>MHVRDTKLTVDDITGVVGIIPTPSIPTADQPGTAFSVDLDEAATLADAMVRGGVDVLMTTGTFGECASLTWDELQSFVATVVDAVAGRIPVFAGATTLNTRDTIARGRRLGELGADGLFVGRPMWLPLDDAGIVRFYRDVAEAVPNMALVVYDNPGAFKGKIGTPAYEALSQIPQVVAAKHLGLLSGSAFLSDLRAVSGRVRLLPLETDWYYFARLFPEEVTACWSGNVACGPAPVTHLRDLIRARRWDDCQALTDELE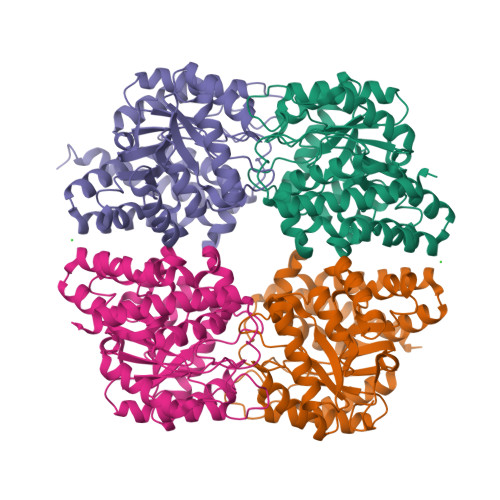GALETLYPGGNFAEFLKYSIQIDNAQFQAAGFMRTGPTRPPYTEVPESYLAGGREAGKNWAALQQRYASLAVSNH[4x]Glycoprotein 2 (GP2) shares a high degree of sequence similarity with UMOD (53% sequence identity), and has been recognized as a paralog of UMOD resulting from gene duplication. GP2 is expressed and secreted by the pancreas and serves a similar antibacterial function in the digestive tract as UMOD does in the urinary tract. Our structure analysis unveiled that GP2 forms filaments with its ZP modules, composing the ZPN and ZPC domains along with a linker that connects these two domains. Our study provides the first experimental evidence of GP2 filament formation and reveals the molecular mechanisms underlying GP2’s adaptation to a different environment compared to UMOD.

In this study, we extracted GP2 filaments from surgically excised human pancreas tissue and determined their cryo-EM structure at 3.5 Å resolution. Cryo-EM data were collected, and analysis of the 2D classes revealed a zigzag-shaped filament species similar to UMOD filaments. In the cryo-EM structure of GP2, the bipartite zona pellucida (ZP) modules (residues 221−478) comprise the filament core. The D10C and EGF-like domains extend outward from the filament core as flexible branches, and no high-resolution densities are observed around these regions. Additionally, two loops on the ZPN domains (residues 239−251 and 264−274) are also flexible and lack well-defined densities, likely because their conformations are influenced by the flexible branch regions. Each ZP module within GP2 filaments is symmetrically related to the adjacent module with a helical twist of approximately 177.2 degrees and a helical rise of approximately 66.3 Å. To form filaments, the ZPN and ZPC domains from a given ZP module are separated by an extended linker (residues 324−348), a ZPC domain from the previous ZP module (ZPC−1), and a ZPN domain from the subsequent ZP module (ZPN+1). These regions assemble through a β-sheet complementation mechanism, where the first and second β-strands in linker region (L1 and L2) complemented the fold of ZPC−1, and the third β-strand in linker region complemented the fold of ZPN+1. The side chain interactions between linker region, ZPC−1, and ZPN+1 are predominantly hydrophobic, with some additional electrostatic interactions. These interactions, alone with five pairs of intra-domain disulfide bonds, contribute to the stability of GP2 filaments, similar to UMOD. We observed extra densities for four N-glycosylation sites on the filament core of GP2 (Asn260, Asn291, Asn342, and Asn362).

>[3x]MPHLMERMVGSGLLWLALVSCILTQASAVQRGYGNPIEASSYGLDLDCGAPGTPEAHVCFDPCQNYTLLDEPFRSTENSAGSQGCDKNMSGWYRFVGEGGVRMSETCVQVHRCQTDAPMWLNGTHPALGDGITNHTACAHWSGNCCFWKTEVLVKACPGGYHVYRLEGTPWCNLRYCTVPRDPSTVEDKCEKACRPEEECLALNSTWGCFCRQDLNSSDVHSLQPQLDCGPREIKVKVDKCLLGGLGLGEEVIAYLRDPNCSSILQTEERNWVSVTSPVQASACRNILERNQTHAIYKNTLSLVNDFIIRDTILNINFQCAYPLDMKVSLQAALQPIVSSLNVSVDGNGEFIVRMALFQDQNYTNPYEGDAVELSVESVLYVGAILEQGDTSRFNLVLRNCYATPTEDKADLVKYFIIRNSCSNQRDSTIHVEENGQSSESRFSVQMFMFAGHYDLVFLHCEIHLCDSLNEQCQPSCSRSQVRSEVPAIDLARVLDLGPITRRGAQSPGVMNGTPSTAGFLVAWPMVLLTVLLAWLF>GSDENYRDIALAFLDESADSGTINAWVNEFAYQGFDPKRIVQLVKERGTAKGRDWKKDVKMMIVLNLVRGNKPEAMMKKMSEKGASIVANLISVYQLKEGNPGRDTITLSRVSAAFVPWTVQALRVLSESLPVSGTTMDAIAGVTYPRAMMHPSFAGIIDLDLPNGAGATIADAHGLFM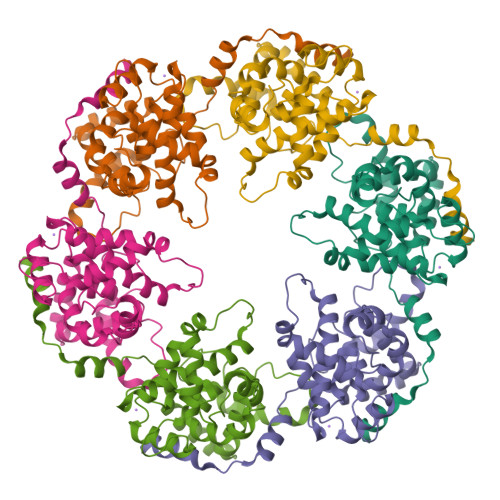IEFSKTINPSLRTKQANEVAATFEKPNMAAMSGRFFTREDKKKLLIAVGIIDEDLVLASAVVRSAEKYRAKVGK[6x]2,5-BIS-O-{3-[AMINO(IMINO)METHYL]PHENYL}-1,4:3,6-DIANHYDRO-D-GLUCITOL | 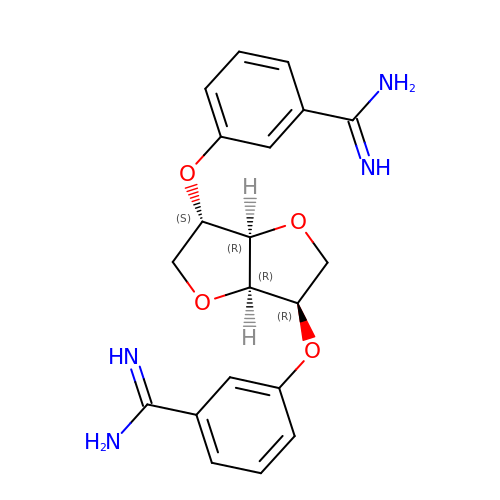C20 H22 N4 O4 | IBIUTOFGXGGVKQ-XMTFNYHQSA-N>[4x]SPSPWDFLGRVLQFQHGDHKRWWDVLAPVFGISMASIGYKLDVQYRHLLVLYDAVIPNMGPFPNSNASNITWTSPFPPGPLEASVNYQAGESSMFRFTIEPVGPHAGTPADPVNELAAKQLMQRLGQLQPGGVDSTMFDHFYPLLCVDGPEARRQWDSIAHIYHKCHTVTALDMQRSAACTLKT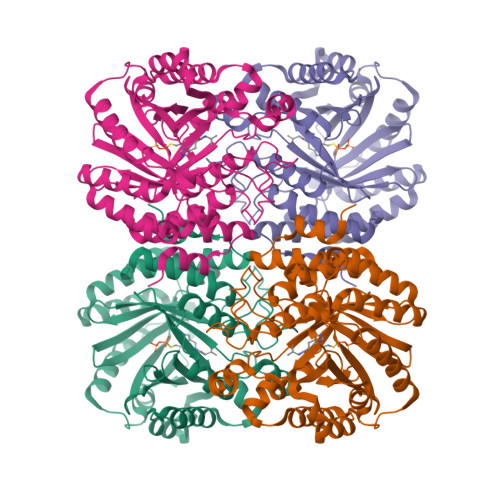YFPPLLRSTIMNTSMVDIMFDAVESFRKQSGLYFDYTKIKEFMSEEKTHETMMVDRSYLSFDCLDPAKSRIKIYTEAKVKTLEEAYSFWSLGGRLSGPEIDYGFKIVSQMWDAIYSKELPGGKQRENNHIQINWEMSAKDSSVAPKLYLTVIEDYDAYVSSAIVDLFTGLGWAAHVQTHKKIEKEAYPMCDANPQSTHAYVWISLAYKKTGPYITVYTNPGASILE>ALTCVMEGKDIEDWSCCPTPWTSFQSSCYFISTGMQSWTKSQKNCSVMGADLVVINTREEQDFIIQNLKRNSSYFLGLSDPGGRRHWQWVDQTPYNENVTFWHSGEPNNLDERCAIINFRSSEEWGWNDIHCHVPQKSICKMK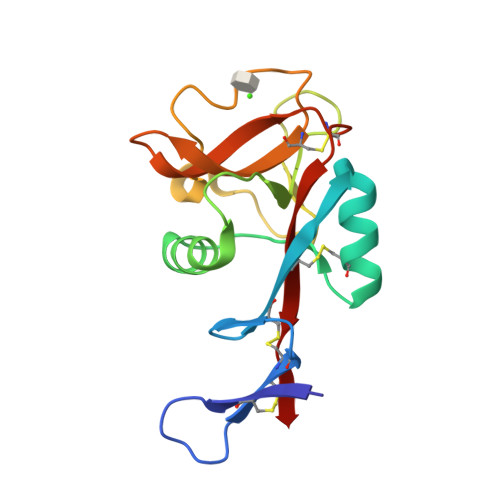KIYI[2x]>PNFSGNWKIIRSENFEELLKVLGVNVMLRKIAVAAASKPA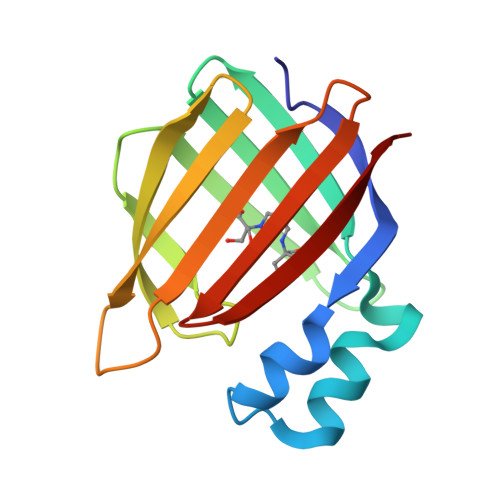VEIKQEGDTFYIKTSTTVETTEINFKVGEEFEEQTVDGRPCKSLVKWESENKMVCEQKLLKGEGPKTSWTLELTNDGELIETMTADDVVCTKVYVRE[2x]> MTAQLQSESTSKIVLVTGGAGYIGSHTVVELIENGYDCVVADNLSNSTYDSVARLEVLTKHHIPFYEVDLCDRKGLEKVFKEYKIDSVIHFAGLKAVGESTQIPLRYYHNNILGTVVLLELMQQYNVSKFVFSSSATVYGDATRFPNMIPIPEECPLGPTNPYGHTKYAIENILNDLYNSDKKSWKFAILRYFNPIGAHPSGLIGEDPLGIPNNLLPYMAQVAVGRREKLYIFGDDYDSRDGTPIRDYIHVVDLAKGHIAALQYLEAYNENEGLCREWNLGSGKGSTVFEVYHAFCKASGIDLPYKVTGRRAGDVLNLTAKPDRAKRELKWQTELQVEDSCKDLWKWTTENPFGYQLRGVEARFSAEDMRYDARFVTIGAGTRFQATFANLGASIVDLKVNGQSVVLGYENEEGYLNPDSAYIGATIGRYANRISKGKFSLCNKDYQLTV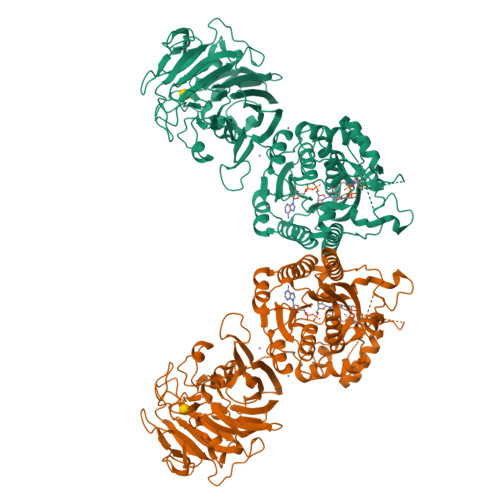NNGVNANHSSIGSFHRKRFLGPIIQNPSKDVFTAEYMLIDNEKDTEFPGDLLVTIQYTVNVAQKSLEIVYKGKLTAGEATPINLTNHSYFNLNKPYGDTIEGTEIMVRSKKSVDVDKNMIPTGNIVDREIATFNSTKPTVLGPKNPQFDCCFVVDENAKPSQINTLNNELTLIVKAFHPDSNITLEVLSTEPTYQFYTGDFLSAGYEARQGFAIEPGRYIDAINQENWKDCVTLKNGETYGSKIVYRFS> MGPKRRQLTF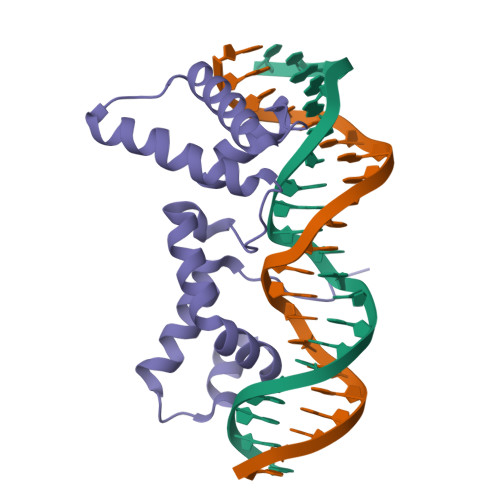REKSRIIQEVEENPDLRKGEIARRFNIPPSTLSTILKNKRAILASERKYGVASTCRKTNKLSPYDKLEGLLIAWFQQIRAAGLPVKGIILKEKALRIAEELGMDDFTASNGWLDRFRRRRS> GPLSLSVDAFKILEDPKWEFPRKNLVLGKTLGEGEFGKVVKATAFHLKGRAGYTTVAVKMLKENASPSELRDLLSEFNVLKQVNHPHVIKLYGACSQDGPLLLIVEYAKYASLRGFLRESRKVGPGYLGSGGSRNSSSLDHPDERALTMGDLISFAWQISQGMQYLAEMKLVHRDLAARNILVAEGRKMKISDFGLSRDVYEEDSYVKRSQGRIPVKWMAIESLFDHIYTTQSDV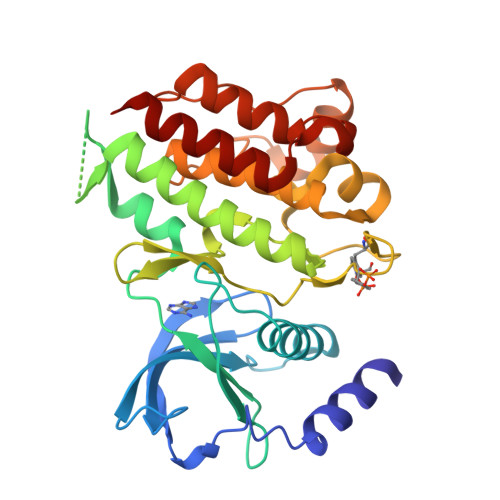WSFGVLLWEIVTLGGNPYPGIPPERLFNLLKTGHRMERPDNCSEEMYRLMLQCWKQEPDKRPVFADISKDLEKMMVKRR>AGITGTWYNQLGSTFIVTAGADGALTGTYESAVGNAESRYVLTGRYDSAPATDGSGTALGWTVAWKNNYRNAHSATTWSGQYVGGAEARINTQW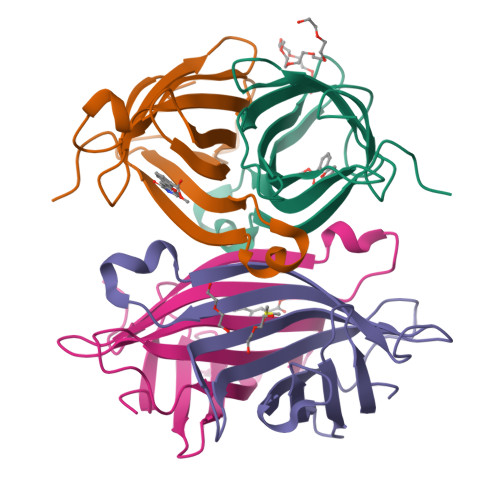LLTSGTTEANAWKSTLVGHDTFTKVKPS[4x]>[6x]MAYTTAQLVTAYTNANLGKAPDAATTLTLDAYATQTQTGGLSDAAALTNTLKLVNSTTAVAIQTYQFFTGVAPSAAGLDFLVDSTTNTNDLNDAYYSKFAQENRFINFSINLATGAGAGATAFAAAYTGVSYAQTVATAYDKIIGNAVATAAGVDVAAAVAFLSRQANIDYLTAFVRANTPFTAAADIDLAVKAALIGTILNAATVSGIGGYATATAAMINDLSDGALSTDNAAGVNLFTAYPSSGVSGSTLSLTTGTDTLTGTANNDTFVAGEVAGAATLTVGDTLSGGAGTDVLNWVQAAAVTALPTGVTISGIETMNVTSGAAITLNTSSGVTGLTALNTNTSGAAQTVTAGAGQNLTATTAAQAANNVAVDGGANVTVASTGVTSGTTTVGANSAASGTVSVSVANSSTTTTGAIAVTGGTAVTVAQTAGNAVNTTLTQADVTVTGNSSTTAVTVTQTAAATAGATVAGRVNGAVTITDSAAASATTAGKIATVTLGSFGAATIDSSALTTVNLSGTGTSLGIGRGALTATPTANTLTLNVNGLTTTGAITDSEAAADDGFTTINIAGSTASSTIASLVAADATTLNISGDARVTITSHTAAALTGITVTNSVGATLGAELATGLVFTGGAGADSILLGATTKAIVMGAGDDTVTVSSATLGAGGSVNGGDGTDVLVANVNGSSFSADPAFGGFETLRVAGAAAQGSHNANGFTALQLGATAGATTFTNVAVNVGLTVLAAPTGTTTVTLANATGTSDVFNLTLSSSAALAAGTVALAGVETVNIAATDTNTTAHVDTLTLQATSAKSIVVTGNAGLNLTNTGNTAVTSFDASAVTGTGSAVTFVSANTTVGEVVTIRGGAGADSLTGSATANDTIIGGAGADTLVYTGGTDTFTGGTGADIFDINAIGTSTAFVTITDAAVGD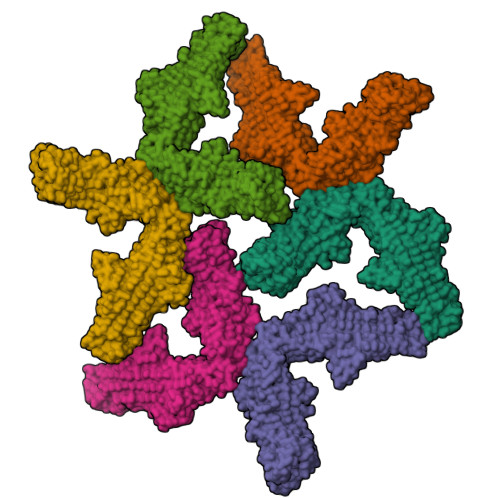KLDLVGISTNGAIADGAFGAAVTLGAAATLAQYLDAAAAGDGSGTSVAKWFQFGGDTYVVVDSSAGATFVSGADAVIKLTGLVTLTTSAFATEVLTLA>[2x]ADTNAPICLCDEPGVLGRTQIVTTEIKDKIEKAVEAVAQESGVSGRGFSIFSHHPVFRECGKYECRTVRPEHSRCYNFPPFTHFKSECPVSTRDCEPVFGYTVAGE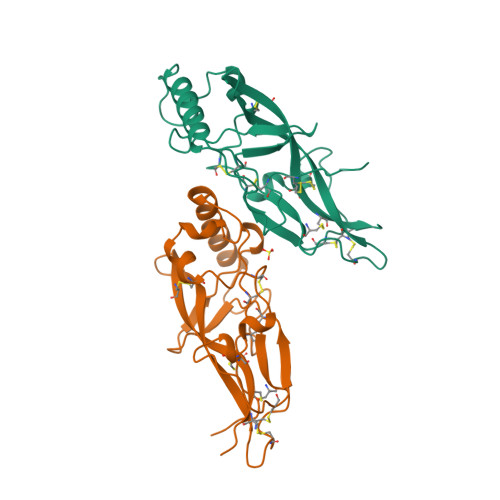FRVIVQAPRAGFRQCVWQHKCRFGSNSCGYNGRCTQQRSVVRLVTYNLEKDGFLCESFRTCCGCPCRSF> MRWGYTSVQGFRDEMEDDIVIRSDAVDSFSYAAVFDGHAGSSSVKFLREELYKECVGALQAGSLLNGGDFAAIKEALIKAFESVDRNLLKWLEANGDEEDESGSTATVMIIRNDVSFIAHIGESCAVLSRSGQIEELTDYHRPYGSSRAAIQEVKRVKEAGGWIVNGRICGDIAVSRAFGDIRFKTKKNDMLKKGVDEGRWSEKFVSRIEFKGDMVVATPDIFQVPLTSDVEFIILASDGLWDYMKSSDVVSY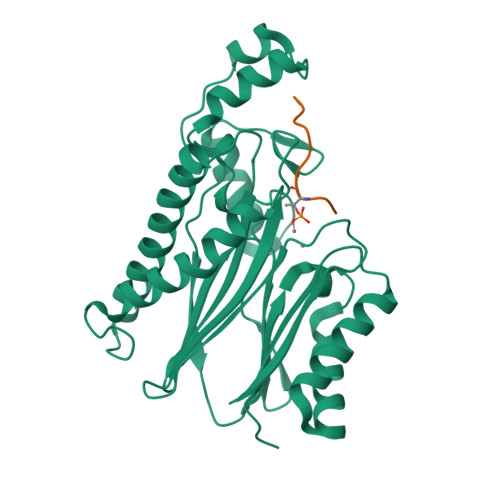VRDQLRKHGNVQLACESLAQVALDRRSQDNISIIIADLGRTLEHHHHHH;> RKTVAKPKGPSGSPW> GDRVADVIESSIGDSVSRALTRALPAPTGQDTQVSSHRLDTGKVPALQAAEIGASSNASDESMIETRCVLNSHSTAETTLDSFFSRAGLVGEIDLPLEGTTNPNGYANWDIDITGYAQMRRKVELFTYMRFDAEFTFVACTPTGQVVPQLLQYMFVPPGAPEPDSRESLAWQTATNPSVFVKLSDPPAQVSVPFMSPASAYQWFYDGYPTFGEHKQEKDLEYGACPNNMMGTFSVRTVGTSKSKYPLVIRIYMRMKHVRAWIPRPMRNQNYLFKANPNYAGNFI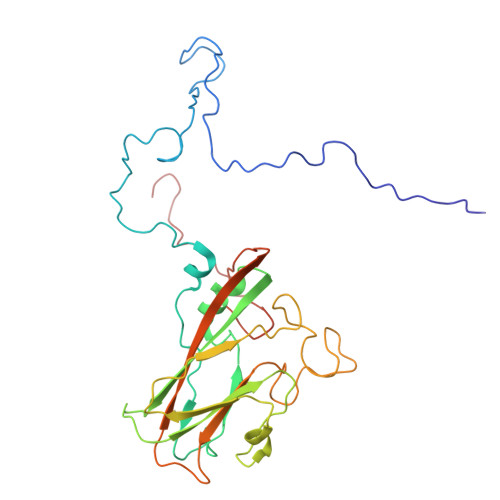KPTGASRTAITTL>[2x]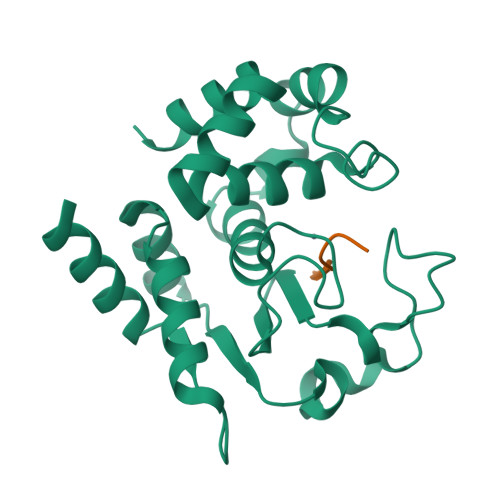GSHMDSTTIQQNKDTLSQIVVFPTGNYDKNEANAMVNRLANIDGKYLNALKQNNLKIKLLSGKLTDEKEYAYLKGVVPKGWEGTGKTWDDVPGLGGSTVALRIGFSNKGKGHDAINLELHATAHAIDHIVLNDISKSAQFKQIFAKEGRSLGNVNFLGVYPEEFFAESFAYYYLNQDTNSKLKSACPQTYSFLQNLAK2-[(2-azanyl-6-oxidanylidene-3,9-dihydropurin-8-yl)sulfanylmethyl]benzenecarbonitrile 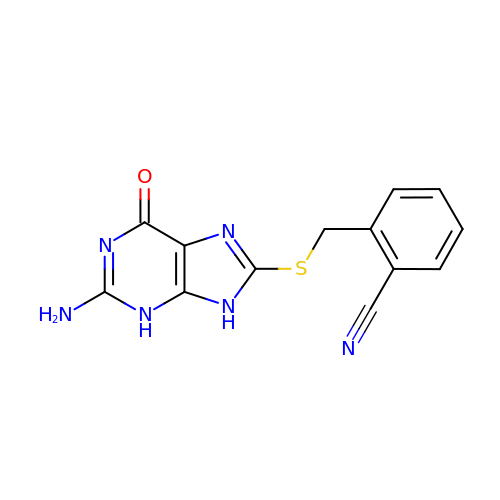| C13 H10 N6 O S | UBLPQTIVHIXXSM-UHFFFAOYSA-N(2R)-2-PHENYL-N-PYRIDIN-4-YLBUTANAMIDE | C15 H16 N2 O | 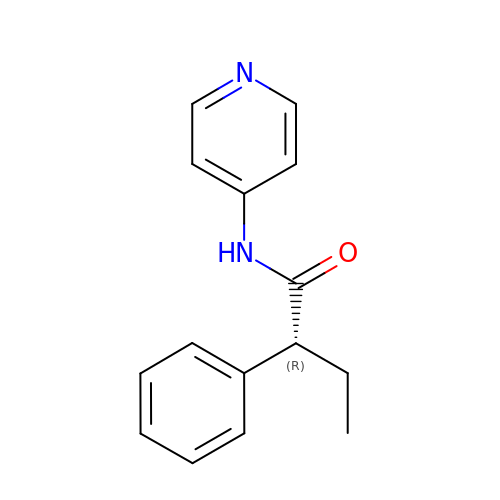MODBYAQUXXEFRM-CQSZACIVSA-N[(2~{R})-3-[[(2~{S})-3-[(2~{S})-2,6-bis(azanyl)hexanoyl]oxy-2-oxidanyl-propoxy]-oxidanyl-phosphoryl]oxy-2-hexadecanoyloxy-propyl] 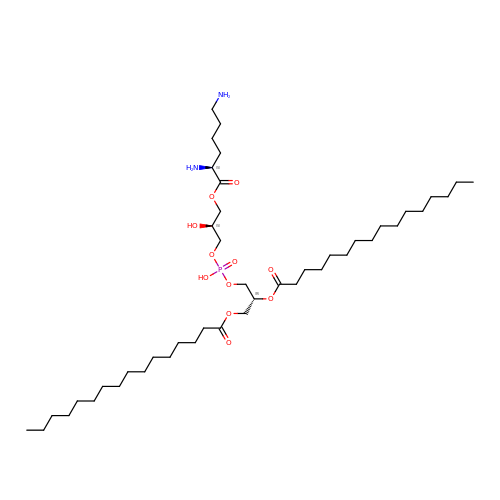hexadecanoate | C44 H87 N2 O11 P | IKYFVWXVCARWQS-HMVVSKLPSA-N>MFSAGHKIKGTVVLMPKNELEVNPDGSAVDNLNAFLGRSVSLQLISATKADAHGKGKVGKDTFLEGINTSLPTLGAGESAFNIHFEWDGSMGIPGAFYIKNYMQVEFFLKSLTLEAISNQG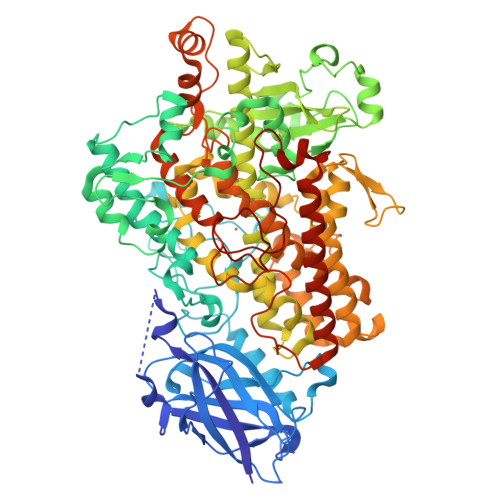TIRFVCNSWVYNTKLYKSVRIFFANHTYVPSETPAPLVEYREEELKSLRGNGTGERKEYDRIYDYDVYNDLGNPDKSEKLARPVLGGSSTFPYPRRGRTGRGPTVTDPNTEKQGEVFYVPRDENLGHLKSKDALEIGTKSLSQIVQPAFESAFDLKSTPIEFHSFQDVHDLYEGGIKLPRDVISTIIPLPVIKELYRTDGQHILKFPQPHVVQVSQSAWMTDEEFAREMIAGVNPCVIRGLEEFPPKSNLDPAIYGDQSSKITADSLDLDGYTMDEALGSRRLFMLDYHDIFMPYVRQINQLNSAKTYATRTILFLREDGTLKPVAIELSLPHSAGDLSAAVSQVVLPAKEGVESTIWLLAKAYVIVNDSCYHQLMSHWLNTHAAMEPFVIATHRHLSVLHPIYKLLTPHYRNNMNINALARQSLINANGAIETTFLPSKYSVEMSSAVYKNWVFTDQALPADLIKRGVAIKDPSTPHGVRLLIEDYPYAADGLEIWAAIKTWVQEYVPLYYARDDDVKNDSELQHWWKEAVEKGHGDLKDKPWWPKLQTLEDLVEVCLIIIWIASALHAAVNFGQYPYGGLIMNRPTASRRLLPEKGTPEYEEMINNHEKAYLRTITSKLPTLISLSVIEILSTHASDEVYLGQRDNPHWTSDSKALQAFQKFGNKLKEIEEKLVRRNNDPSLQGNRLGPVQLPYTLLYPSSEEGLTFRGIPNSISI[2x]> GMKNLLGYSEDYLKERKGYITAKEICNQPKLWRETYEIILSQREKLKSFLDNFAKKPNAKIVITGAGSSAFVGNSVVSYLNAKENIKIEAIATTDIVSHPFYYLKKDEPTLLISCARSGNSPESTAAVTLAEKIVDDISHLIITCNSEGKLALHAKRNYNSFLLLMPEESNDKGFAMTGSFSTMLLS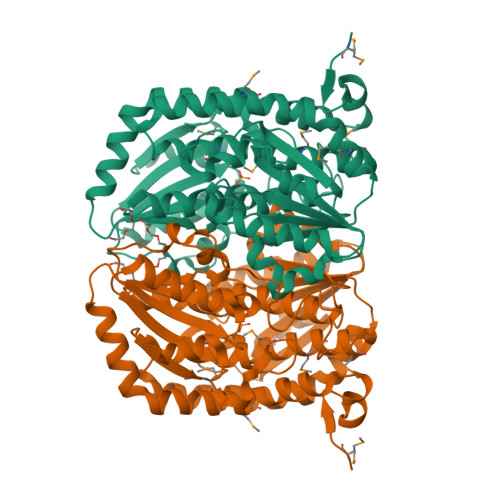CLLIFNLDKLESIGKQIESISMQGEKVLVNNVELMKKIVGEKFKRTVYLGAANAFGLAKESALKVLELTAGKIATLYDTPLGFRHGPKSIIDDETLIVIFFSNDTYAREYEYDLLKEVYSQNGNHKVLAISEYEDKLIEDNSDYFIAINKEEQEYEDDSFLSLDYLLNAQMYAFINSMELGIGPDNPCPTGEVNRVVKGVIIHDYR>[24x]MANPTLFVSYDQNGKKLSFANWISVLSPQDTPFVSMTGKESINQTIFSWQTDALASVDGNNAHVEGSRAEDGEMKPTVIKSNVTQILRKVVRVSDTANTTANYGRGRELMYQLEKKGKEIKRDLEKILLSGQARTDVLADQYLTNSAADPAVAGLNDTHAARKTGAFQFLCAHGGLAGG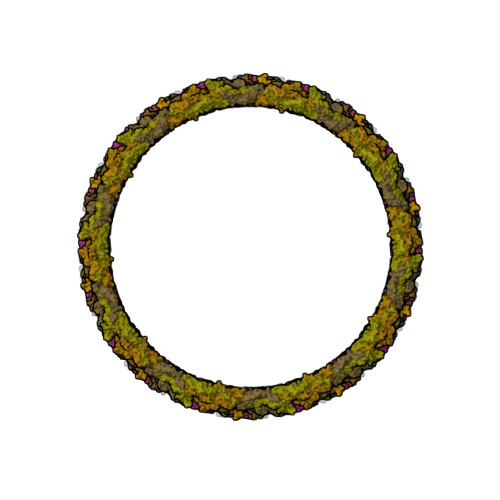VVDKTKNGPADPDTGAVTVKVAQNASNPTTNIGFDEADIFDMTLQLYTAGSEADIIMINPAHAKIFAGLQENTQGSRKRIFENTKQFIYEVNSITDPLGQSYKIIVNRWMPTDAVYFFRSADWTQMVLRAPKRTELAKDGSYEKWMIEMEVGLRHRNPYASGVLFTAAGKAAA>MLSFLLTLKRMLRACLRAWKDKEFQVLFVLTILTLISGTIFYSTVEGLRPIDALYFSVVTLTTVGAGNFS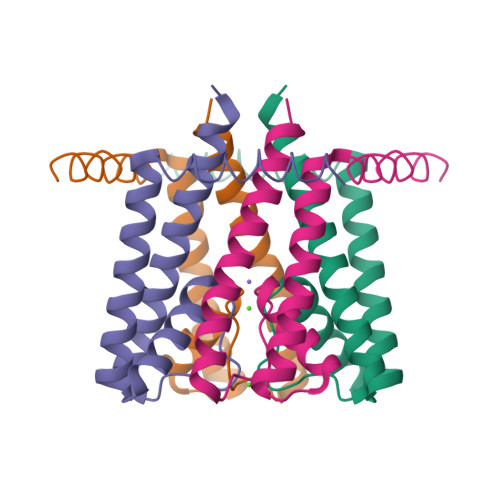PQTDFGKIFTILYIFIGIGLVFGFIHKLAVNVQLPSILSNLVPR[2x]In this study, a PETase-like enzyme (PETase SM14) from Streptomyces sp. SM14 was heterologously produced in Escherichia coli, and its activity was tested on post-consumer plastic substrates using high-performance liquid chromatography for product quantification as well as scanning electron microscopy and atomic force microscopy for substrate surface imaging evaluation. PETase SM14 exhibited high salt tolerance (1.5 M), good heat resistance (Tm 56.26 °C), and optimal activity at pH 9.0, highlighting its potential for PET waste bioremediation. All three enzymes share conserved motifs, including the serine hydrolase sequence Gly-x1-Ser-x2-Gly and the catalytic triad Ser-Asp-His. Due to its thermostability and activity on PCP, PETase SM14 may represent an interesting tool for enzymatic PET waste management.

Furthermore, its X-ray crystal structure was solved at 1.43 Å resolution, revealing conserved features of the PETase family with potential relevance for future engineering applications. The X-ray structure of PETase SM14 (UniProt ID: A0A679PDB4) validated the accuracy of the predicted AlphaFold structure, exhibiting a high structural identity with a root-mean-square deviation (RMSD) of 0.278 Å. Notably, this extends to the loop regions, where the catalytic site is located. Structural alignment of the three enzymes shows a high degree of similarity, with an RMSD of 0.691 Å across 190 Cα atoms for IsPETase and an RMSD of 0.81 Å over 195 Cα atoms for PE-H including the catalytic triad within the active site pocket. The catalytic triad of PETase SM14 (blue sticks) comprises S156, D202, and H234, while that of IsPETase (green sticks) includes S160, D206, and H237 and S171, D217, and H249 for PE-H from P. aestusnigri (pink sticks). While the catalytic residues align across all three, the catalytic pocket appears more closed in PE-H and SM14 compared to that in IsPETase. For instance, Y88 and F98 in PETase SM14 and PE-H, respectively, are positioned in such a way that the catalytic pocket appears to be more closed. Structural alignment enabled the identification of the corresponding residues of PETase SM14 and PE-H, which have a nearly identical arrangement: Y88, H155, M157, W181, I204 and F98, W170, M172, W195, and I219. In PETase SM14, however, the motif includes a histidine (H155), instead of a tryptophan (W159), which is commonly found in IsPETase and related hydrolases, ,, also in PE-H (W170). IsPETase features a highly polarized surface charge, resulting in an isoelectric point (pI) of 9.41, whereas PETase SM14 and PE-H have a theoretical pI of 6.67 and 6.54, respectively (as determined by the ExPASy, ProtParam tool), and both exhibit a less polarized and more delocalized surface charge.

> GWELQAQNPHERGPDPSNSYIEQARGSYSVSQRSISRLGSDGFRDGTMYYPTSTADGRFGVVAISPGYTASESTIAWLGPRLASFGFVVVTINTDSRYDQPRQRATQLHAALDHAIGDSVVGPRIDTSRQAVMGHSMGGGGALQAAEERDEIRAAVPLTPWNLKKGWSGVDAATLVIGAENDAIAPVRSHSIPFYESLTNAERRAYLELRREGHFAPNSSNTLIAKYSVSWLKRYVDNDLRYDQFIDPGPRTGITTGVSDYRLG>[34x]MWRLRRAAVACEVCQSLVKHSSGIKGSLPLQKLHLVSRSIYHSHHPTLKLQRPQLRTSFQQFSSLTNLPLRKLKFSPIKYGYQPRRNFWPARLATRLLKLRYLILGSAVGGGYTAKKTFDQWKDMIPDLSEYKWIVPDIVWEIDEYIDFEKIRKALPSSEDLVKLAPDFDKIVESLSLLKDFFTSGSPEETAFRATDRGSESDKHFRKVSDKEKIDQLQEELLHTQLKYQRILERLEKENKELRKLVLQKDDKGIHHRKLKKSLIDMYSEVLDVLSDYDASYNTQDHLPRVVVVGDQSAGKTSVLEMIAQARIFPRGSGEMMTRSPVKVTLSEGPHHVALFKDSSREFDLTKEEDLAALRHEIELRMRKNVKEGCTVSP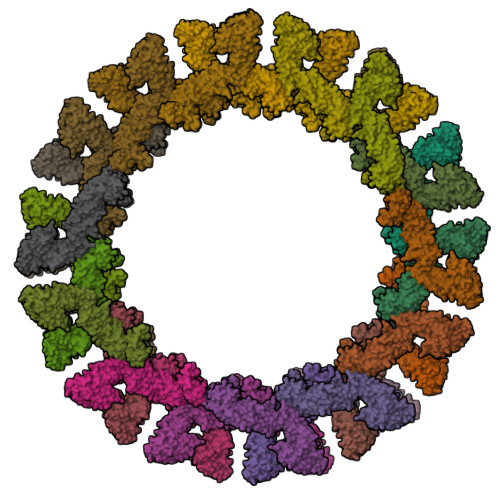ETISLNVKGPGLQRMVLVDLPGVINTVTSGMAPDTKETIFSISKAYMQNPNAIILCIQDGSVDAERSIVTDLVSQMDPHGRRTIFVLTKVDLAEKNVASPSRIQQIIEGKLFPMKALGYFAVVTGKGNSSESIEAIREYEEEFFQNSKLLKTSMLKAHQVTTRNLSLAVSDCFWKMVRESVEQQADSFKATRFNLETEWKNNYPRLRELDRNELFEKAKNEILDEVISLSQVTPKHWEEILQQSLWERVSTHVIENIYLPAAQTMNSGTFNTTVDIKLKQWTDKQLPNKAVEVAWETLQEEFSRFMTEPKGKEHDDIFDKLKEAVKEESIKRHKWNDFAEDSLRVIQHNALEDRSISDKQQWDAAIYFMEEALQARLKDTENAIENMVGPDWKKRWLYWKNRTQEQCVHNETKNELEKMLKCNEEHPAYLASDEITTVRKNLESRGVEVDPSLIKDTWHQVYRRHFLKTALNHCNLCRRGFYYYQRHFVDSELECNDVVLFWRIQRMLAITANTLRQQLTNTEVRRLEKNVKEVLEDFAEDGEKKIKLLTGKRVQLAEDLKKVREIQEKLDAFIEALHQEK>[4x]MA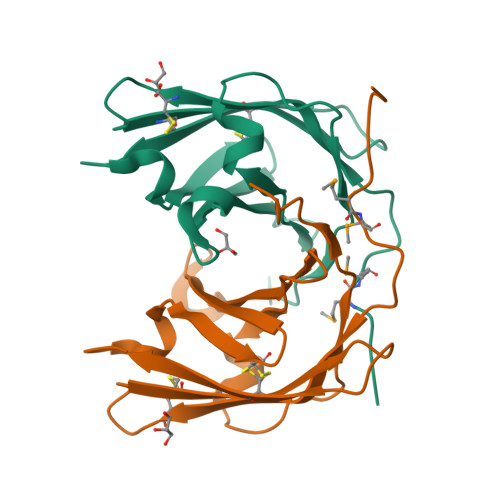APTPADKSMMAAVPEWTITNLKRVCNAGNTSCTWTFGVDTHLATATSCTYVVKANANASQASGGPVTCGPYTITSSWSGQFGPNNGFTTFAVTDFSKKLIVWPAYTDVQVQAGKVVSPNQSYAPANLPLEHHHHHH> AQIPESAKAVVVLSPYSLQHVFPREWVTKSYRKTIVERPERLLASSMGISAAITMYPSLFTLKSSHQRKGSLMAPHVLKVHGSSWPAELIELCQMADAKLLKGEIEVPDTWNSGDIYLSSKTIKALQGTIGAIETGVDSIFKGPSAEHISNRA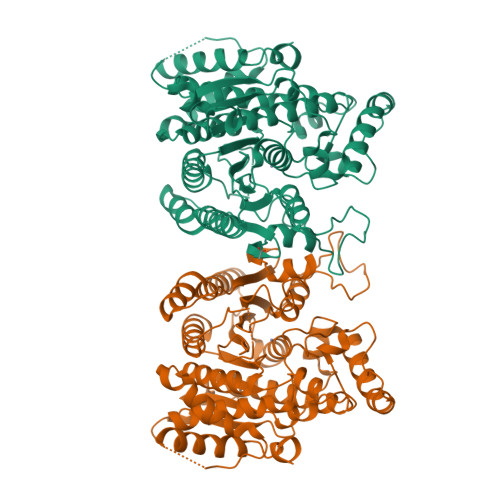FVAIRPPGHHCHYGTPSGFCLLNNAHVAIEYAYDTYNVTHVVVLDFDLHHGDGTQDICWKRAGFKPEEEPEDSSYDDFGKKFAEFPKVGYFSMHDINSFPTESGFATKENIKNASTCIMNSHDLNIWNIHLSKWTTEEEFNVLYRTKYRTLFAKADEFFRSAKLEMNQQGRPFKGLVVISAGFDASEFEQTSMQRHSVNVPTSFYTTFTKDALKLAQMHCHGKVLSLMEGGYSDKAICSGVFAHLIGLQNQDWVKEWGSEQVVKEIVRGCKPAWKPYKTKRAKDVIRIWAEEVIRLGRAMIPEFDDIIFKDAVNSAPSNSLLKA>SPRGLELLIAQTILQGFDAQYGRFLEVTSGAQQRFEQADWHAVQQAMKNRIHLYDHHVGLVVEQLRCITNGQSTDAEFLLRVKEHYTRLLPDYPRFEIAESFFNSVYCRLFDHRSLTPERLFIFSSQPERRFRTIPRPLAKDFHPDHGWESLLMRVISDLPLRLHWQNKSRDIHYIIRHLTETLGPENLSKSHLQVANELFYRNKAAWLVGKLITPSGTLPFLLPIHQTDDGELFIDTCLTTTAEASIVFGFARSYFMVYAPLPAALVEWLREILPGKTTAELYMAIGCQKHAKTESYREYLVYLQG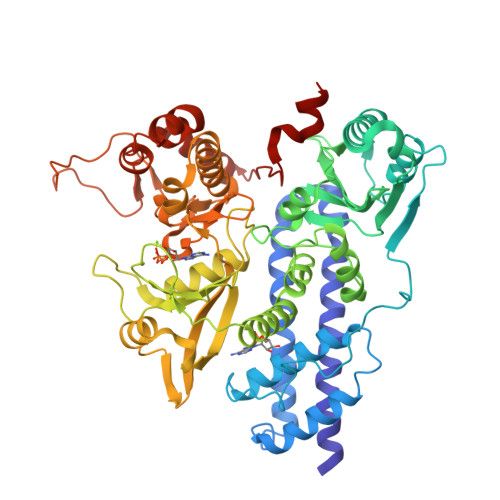CNEQFIEAPGIRGMVMLVFTLPGFDRVFKVIKDKFAPQKEMSAAHVRACYQLVKEHDRVGRMADTQEFENFVLEKRHISPALMELLLQEAAEKITDLGEQIVIRHLYIERRMVPLNIWLEQVEGQQLRDAIEEYGNAIRQLAAANIFPGDMLFKNFGVTRHGRVVFYDYDEICYMTEVNFRDIPPPRYPEDELASEPWYSVSPGDVFPEEFRHWLCADPRIGPLFEEMHADLFRADYWRALQNRIREGHVEDVYAYRRRQRFSVRYGEMLF[2x]Keratinases are classified in the superfamily of subtilisin-like proteases, belonging to the serine protease (S8 family). In this study, we identified a thermostable keratinase (MtaKer) from the thermophile strain, Meiothermus taiwanensis WR-220, which grows at 55–65 °C11. Like many subtilisin-like serine proteases, bioinformatic analysis indicates that Mtai_v1c14470 consists of three parts, including signal peptide, N-terminal pro-peptide (N-pro), and mature protease, and has the three highly conserved catalytic triad residues Asp39, His72, and Ser224. Unlike most reported keratinases, which are only active at pH 6–9 and temperatures 25–50 °C4, 8, rMtaKer has keratinolytic activities at temperatures ranging from 25 to 75 °C and pH from 4 to 11, with the optimal temperature and pH at 65 °C and pH 10.

The crystal structure of mature rMtaKer was determined at a resolution of 1.50 Å and contained three monomers in an asymmetric unit. Each monomer consists of the central seven-stranded parallel β sheets flanking by six α helices and four β sheets made of two anti-parallel strands and possesses the conserved catalytic triad Asp39, His72 and Ser224. Two calcium ions and two disulfide bridges were also found in the structure of rMtaKer. The first calcium ion (1Ca), involved in stabilizing the surface loop between α1 and β2, is coordinated by Oδ1 of Asp11 and Asp14, carbonyl-oxygen of Asp11 and Thr23, Oγ of Ser21, Oε of Gln15, and one water molecule in a pentagonal bipyramidal manner. The second calcium (2Ca) makes contact with the main-chain carbonyl oxygen atoms of the Val172, Gly175, Thr177, and two water molecules. The first disulfide bond, Cys69-Cys101, connects the loops which are involved in substrate-binding. The second disulfide bond, Cys165-Cys196, is close to the 2Ca-binding site and the region carrying residues of the S1 active-site pocket, which was termed S1–S4 according to a previous report. Each C-terminus His-tag protrudes into the adjacent monomer as a substrate, resulting the unexpected His-tag removal at Tyr278. The remaining residues at the C-terminal end (Tyr278-Glu279-Asn280-Leu281-Tyr282) of rMtaKer was buried in the active-site cavity of the adjacent subunit. Our crystal structure clearly shows that Ser224 acts as a nucleophile to attack the carbonyl carbon of the scissile peptide bond on Tyr282 and forms a tetrahedral acyl enzyme intermediate which can be stabilized by the oxyanion hole of Asn159 and Thr223.

>ATQTGATWGLDRIDQRTLPLSGTFTYSNTGSGVNAYIIDTGIRVSHSEFGGRATAVFDAIGDGQNGNDCNGHGTHVAGTVGGTVYGVAKSVRLYAVRVLNCSGSGSNSGVIAGVDWVRQNARRPAVANMSLGGGASSALDTAVNNAINAGITFALAAGNSNRDACQFSPARVTAGITVGATTSTDARASYSNYGSCLDLFAPGSSITSAWISSDTSTNTISGTSMATPHVAGVAALYLQSNPSASPATVRNAIVGNATSGVVSNAGRRSPNLLLYSNYENLYFQSHHHHHHWSHPQFEK[3x]>[2x]CG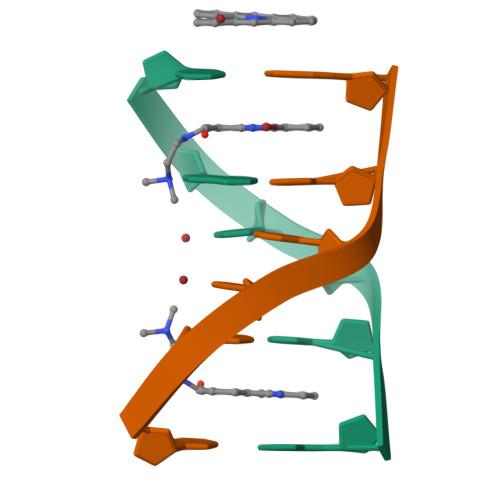UACG> DPNRAPPCDSSQCVLPDCFCSEDGTVIPGDLPARDVPQMITITFDDAINNNNIELYKEIFNGKRKNPNGCDIKATYFVSHKYTNYSAVQETHRKGHEIAVHSITHNDDERFWSNATVDDWGKEMAGMRVIIEKFSNITDNSVVGVRAPYLRVGGNNQFTMMEEQAFLYDSTITAPLSNPPLWPYTMYFRMPHRCHGNLQSCPTRSHAVWEMVMNELDRREDPSNDEYLPGCAMVDSCSNILTGDQFYNFLNHNFDRHYEQNRAPLGLYFHAAWLKNNPEFLEAFLYWIDEILQSHNDVYFVTMTQVIQWVQNPRTVTEAKNFEPWREKCSVEGNPACWVPHSCKLTSKEVPGETINLQTCLR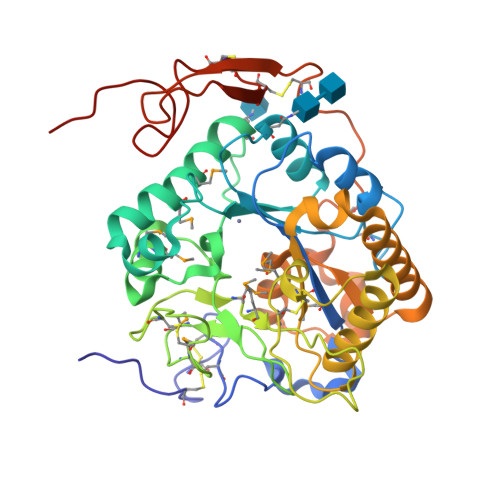CPVNYPWLNDPTGDGHYHHHHHH>GLSAEQIAVLQEQGFELRDEGWEFGMSSKVLFGNNLDRLNPDSRNTLTKIARALL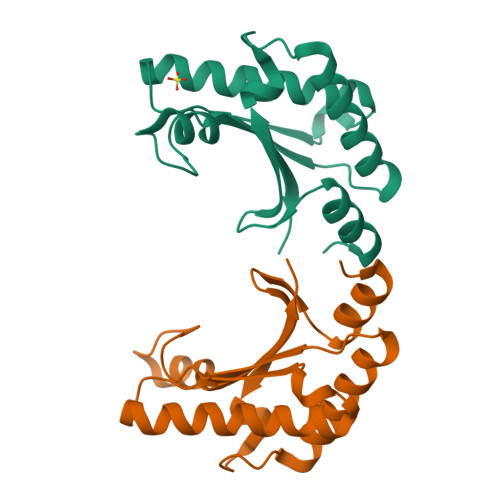AVDIDKVRLEGHTDNYGDEGYNQKLSERRAESVAAVFREAGMPAANIEVRGLGMSKPVADNKTRAGRSENRRVAIIVPAE[4x]> MKTKPLPTAPMAWAESAVETTTSPRELAGHAPLRRVLRPPIARRDGPVLLGDRAPRRTASTMWLLGIDPAESSPGTRATRDDTEQAVDKILRGARRAGGLTVPGAPRYHLTRQVTLTDLCQPNAERAGALLLALRHPTDLPHLARHRAPPGRQTERLAEAWGQ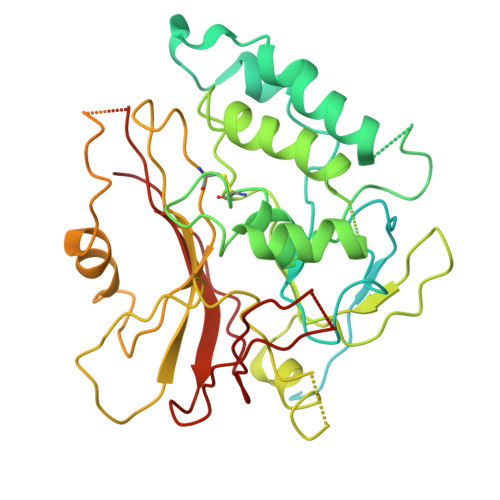LLEASALGSGRAESGCARAGLVSFNFLVAACAAAYDARDAAEAVRAHITTNYGGTRAGARLDRFSECLRAMVHTHVFPHEVMRFFGGLVSWVTQDELASVTAVCSGPQEATHTGHPGRPRSAVTIPACAFVDLDAELCLGGPGAAFLYLVFTYRQCRDQELCCVYVVKSQLPPRGLEAALERLFGRLRITNTIHGAEDMTPPPPNRNVDFPLAVLAASSQSPRCSASQVTNPQFVDRLYRWQPDLRGRPTARTCTYAAFAELGVMPDDSPRCLHRTERFGAVGVPVVILEGVVWRPGGWRACA> MGSSHHHHHHSQDPSEIWRQCKGERHIRPLQGRLVRLVESQEQVATLQLVDTLEEQALLEELLESSKPPVPADAEPLHYLLKTPFRYPPLRWGSRFGRRHEPSLFYAALKLETAMAESAYYRCVLWSGMVVPPPSGRILSEHASFEAGWKVERGIRLQAPPFSDHEAALTDIADYRAPQELGSAMRSAGVQAFEYRSARCPERGCNVALFTPAAF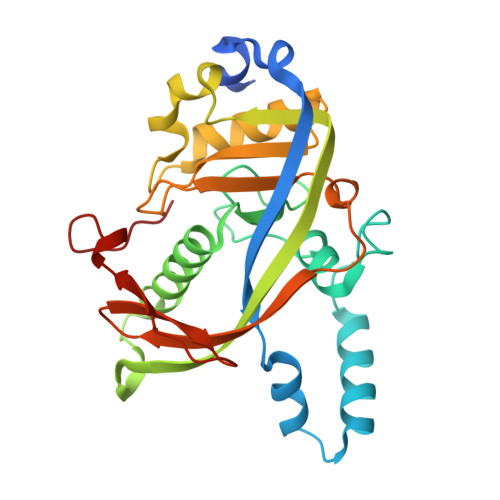TEKRPRNLTPWLCETTAGYVAFKPAHVPGSPKIFSWELFLVDGKLPHPA> GAMDPSEALQRPVASDFEPQGLSEAARWNSKENLLAGPSENDPNLFVALYDFVASGDNTLSITKGEKLRVLGYNHNGEWCEAQTKNGQGWVPSNYITPVNSLEKHSWYHGPVSRNAAEYLLSSGINGSFLVRESESSPGQRSISLRYEGRVYHYRINTASDGKLYVSSESRFNTLAELVHHHSTVADGLITTLHYPAPKRNKPTVYGVSPNYDKWEMERTDITMKHKLGGGQYGEVYEGVWKKYSLTVAVKTLKEDTMEVEEFLKEAAVMKEIKHPNLVQLLGVCTREPPFYIIIEFMTYGNLLDYLRECNRQEVNAVVLLYMATQISSAMEYLEKKNFIHRNLAARNCLVGENHLVKVADFGLSRLMTGDTYTAHAGAKFPIKWTAPESLAYNKFSIKSDVWAFGVLLWEIA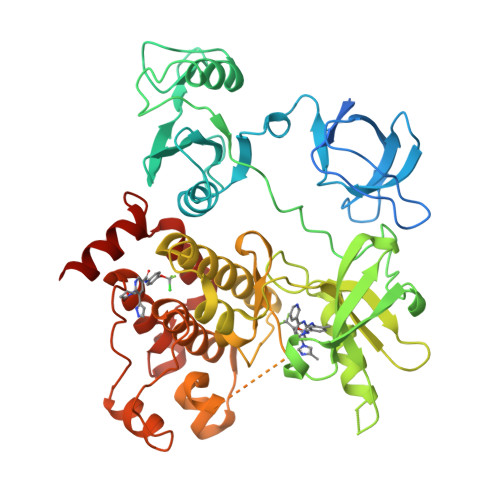TYGMSPYPGIDLSQVYELLEKDYRMERPEGCPEKVYELMRACWQWNPSDRPSFAEIHQAFETMFQESSISDEVEKELGKQGV> SLQDPCSNCPAGTFCDNNRNQICSPCPPNSFSSAGGQRTCDICRQCKGVFRTRKECSSTSNAECDCTPGFHCLGAGCSMCEQDCKQGQ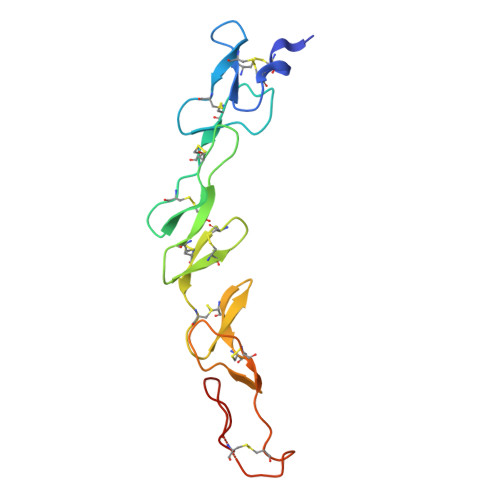ELTKKGCKDCCFGTFNDQKRGICRPWTNCSLDGKSVLVNGTKERDVVCGP>[2x]MAGLNDIFEAQKIEWHEMAGKKVLIVYAHQEPKSFNGSLKNVAVDELSRQGCTVTVSD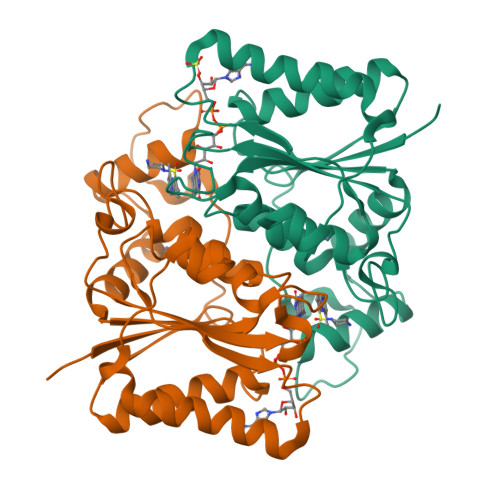LYAMNFEPRATDKDITGTLSNPEVFNYGVETHEAYKQRSLASDITDEQKKVREADLVIFQFPLYWFSVPAILKGWMDRVLCQGFAFDIPGFYDSGLLQGKLALLSVTTGGTAEMYTKTGVNGDSRYFLWPLQHGTLHFCGFKVLAPQISFAPEIASEEERKGMVAAWSQRLQTIWKEEPIPCTAHWHFGQ>MSGNTYGKLFTVTTAGESHGPALVAIVDGCPPGLELSARDLQRDLDRRKPGTSRHTTQRQEADEVEILSGVFEGKTTGTPIGLLIRNTDQKSKDYSAIKDLFRPAHADY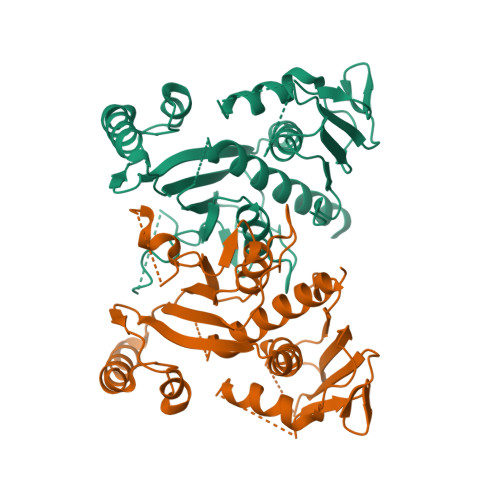TYHHKYGVRDYRGGGRSSARETAMRVAAGAIAKKYLAGLGIQVRGYMSQLGPIEIPFRSWDSVEQNAFFSPDPDKVPELEAYMDQLRRDQDSVGAKITVVAEGVPPGLGEPIFDRLDAELAHALMSINAVKGVEIGAGFASIAQRGTEHRDELTPQGFLSNNAGGILGGISSGQPIVAHLALKPTSSITTPGRSIDTAGEPVDMITKGRHDPCVGIRATPIAEAMMAIVLLDQLLRQRGQNADVRVDTPVLPQL[2x]>MRGSHHHHHHGSIRDDFLRLPSQASKFFQADDNVEGTRWAVLVAGSKGYVNYRHQADVCHAYQILKKGGLKDENIIVFMYDDIAYNESNPHPGVIINHPYGSDVYKGVPKDYVGEDINPPNFYAVLLANKSALTGTGSGKVLDSGPNDHVFIYYTNHGGAGVLGMPSKPYIAASDLNDVLKKKHASGTYKSIVFYVESCESGSMFDGLLPEDHNIYVMGASDTGESSWVTYCPLQHPSPPPEYDVCVGDLFSVAWLEDCDVHNLQTETFQQQYEVVKNKTIVALIEDGTHVVQYGDVGLSKQTLFVYMGTDPANDNNTFTDKNSLGTPRKAVSQRDADLIHYWEKYRRAPEGSSRKAEAKKQLREVMAHRMHIDNSVK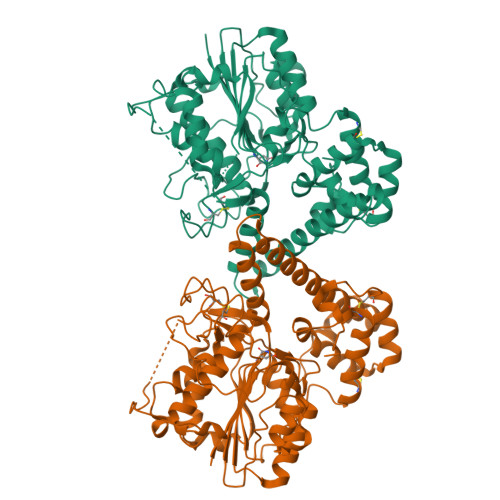HIGKLLFGIEKGHKMLNNVRPAGLPVVDDWDCFKTLIRTFETHCGSLSEYGMKHMRSFANLCNAGIRKEQMAEASAQACVSIPDNPWSSLHAGFS[4x]>[2x]HMERLLDELTLEGVARYMQSERCRRVICLVGAGISTSAGIPDFRSPSTGLYDNLEKYHLPYPEAIFEISYFKKHPEPFFALAKELYPGQFKPTICHYFMRLLKDKGLLLRCYTQNIDTLERIAGLEQEDLVEAHGTFYTSHCVSASCRHEYPLSWMKEKIFSEVTPKCEDCQSLVKPDIVFFGESLPARFFSCMQSDFLKVDLLLVMGTSLQVQPFASLISKAPLSTPRLLINKEK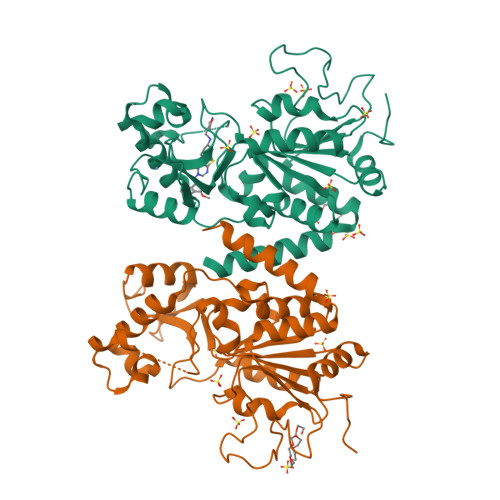AGQSDPFLGMIMGLGGGMDFDSKKAYRDVAWLGECDQGCLALAELLGWKKELEDLVRREHASIDAQS> KWYYKTITFLPELCNNESLAAKCLRVLHGFNYQYETRNIGVSFPLWCDATVGKKISFVSKNKIELDLLLKQ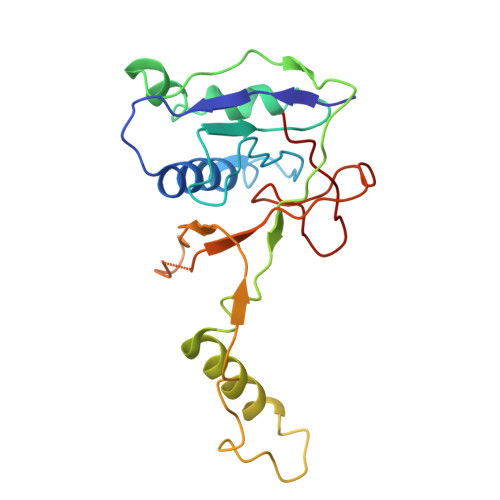HYFVQMEQLQYFHISNTVLVPEDCTYVSFRRCQSIDKLTAAGLARKIRRLEKRALSRGEQFDPSSFAQKEHTAIAHYHSLGESSKQTNRNFRLNIRMLSEQPREGNSIFSSYGLSNSENSFQPVPLI> MTNTLQVKLLSKNARMPERNHKTDAGYDIFSAETVVLEPQEKAVIKTDVAVSIPEGYVGLLTSRSGVSSKTHLVIETGKIDAGYHGNLGINIKNDHEDDKMQTIFLRNIDNEKIFEKERHLYKLGSYRIEKGERIAQLVIVPIWTPELKQVEEFESVSERGEKGFG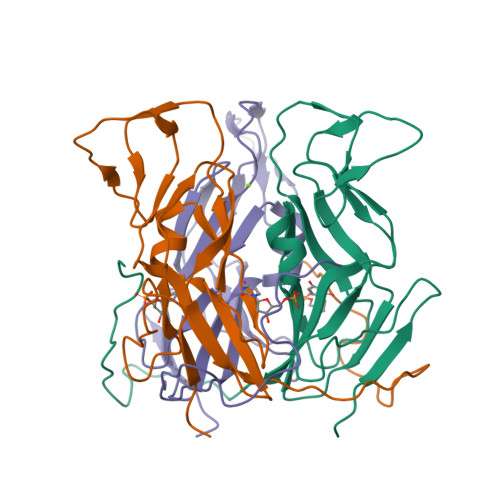SSGV> MGVALGATRVIYPAGQKQEQLAVTNNDENSTYLIQSWVENADGVKDGRFIVTPPLFAMKGKKENTLRILDATNNQLPQDRESLFWMNVKAIPSMDKSKLTENTLQLAIISRIKLYYRPAKLALPPDQAAEKLRFRRSANSLTLINPTPYYLTVTELNAGTRVLENALVPPMGESTVKLPSDAGSNITYRTINDYGALTPKMTGVMEHHHHHH;> DLYFNPRFLADDPQAVADLSRFENGQELPPGTYRVDIYLNNGYMATRDVTFNTGDSEQGIVPCLTRAQLASMGLNTASVAGMNLLADDACVPLTTMVQDATAHLDVGQQRLNLTIPQAFMSNRARGYIPPELWDPGINAGLLNYNFSGNSVQNRIGGNSHYAYLNLQSGLNIGAWRLRDNTTWSYNSSDRSSGSKNKWQHINTWLERDIIPLRSRLTLGDGYTQGDIFDGINFRGAQLASDDNMLPDSQRGFAPVIHGIARGTAQVTIKQNGYDIYNSTVPPGPFTINDIYAAGNSGDLQVTIKEADGSTQIFTVPYSSVPLLQREGHTRYSITAGEYRSGNAQQEKPRFFQSTLLHGLPAGWTIYGGTQLADRYRAFNFGIGKNMGALGALSVDMTQANSTLPDDSQHDGQSVRFLYNKSLNESGTNIQLVGYRYSTSGYFNFADTTYSRMNGYNIETQDGVIQVKPKFTDYYNLAYNKRGKLQLTVTQQLGRTSTLYLSGSHQTYWGTSNVDEQFQAGLNTAFEDINWTLSYSLTKNAWQKGRDQMLALNVNIPFSHWLRSDSKSQWRHASASYSMSHDLNGRMTNLAGVYGTLLEDNNLSYSVQTGYAGGGDGNSGSTGYATLNYRGGYGNANIGYSHSDDIKQLYYGVSGGVLAHANGVTLGQPLNDTVVLVKAPGAKDAKVENQTGVRTDWRGYAVLPYATEYRENRVALDTNTLADNVDLDNAVANVVPTRGAIVRAEFKARVGIKLLMTLTHNNKPLPFGAMVTSESSQSSGIVADNGQVYLSGMPLAGKVQVKWGEEENAHCVANYQLPPESQQQLLTQLSAECRLVPRGSWSHPQFEK;> GNKWNTTLPGGNMQFQGVIIAETCRIEAGDKQMTVNMGQISSNRFHAVGEDSAPVPFVIHLRECSTVVSERVGVAFHGVADGKNPDVLSVGEGPGIATNIGVALFDDEGNLVPINRPPANWKRLYSGSTSLHFIAKYRATGRRVTGGIANAQAWFSLTYQ

Uropathogenic Escherichia coli strains use filamentous type 1 pili to adhere to and invade uroepithelial cells. The pilus consists of a flexible tip fibrillum, formed by the adhesin FimH and the subunits FimG and FimF. The pilus rod is a helical assembly of up to 3000 copies of the main subunit FimA, terminated by a single copy of the subunit FimI that anchors the rod to the assembly platform FimD in the outer membrane. The assembly platform FimD in the outer membrane of uropathogenic E. coli is the catalyst of type 1 pilus assembly.

To explore the structural implications of FimI-mediated termination of pilus assembly, we performed a FimD-catalyzed assembly reaction of pilus rods in vitro similar to the one for the FimDHGFAnC complex, except that excess FimICHis was also added at the end of the reaction. Using Ni-NTA affinity chromatography, we separate complexes with a terminal FimICHis subunit from complexes with terminal FimAnC and determine the structure of the FimI-terminated assembly platform at 3.6 Å resolution (map XIII). To identify structural parameters explaining assembly termination by FimI, we next analyzed the interfaces between FimC and FimA (model IV), FimC and FimI (model XIII), and FimC and FimF (PDB-ID 6E1422) in the respective FimD complexes. While the interactions between FimC and the respective subunit (FimA, FimI, FimF) are primarily mediated through backbone hydrogen bonding involving the G1 strand of FimC, differences emerge in the interactions with FimA strand A’. In contrast to FimA and FimF, FimI does not only form hydrogen bonds with the neighboring A1’ strand of FimC, but also with the B1 strand of FimC. Here, Arg25 of FimI additionally interacts with Thr23 and Asn25 of the B1 strand of FimC via hydrogen bonds. In general, the total interface area between FimI and FimC (1739 Å2) is larger than that of FimA and FimC (1562 Å2) or FimF and FimC (1449 Å2) and involves more potential hydrogen bonds (FimI-FimC: 30 H-bonds, FimA-FimC: 21 H-bonds, FimF-FimC: 19 H-bonds). Indeed, we also identified a closed P5 pocket in the FimD-bound FimIC complex. However, when comparing the usher complexes with FimA or FimI as the last incorporated subunit with the usher-tip fibrillum complex (last subunit: FimF, with open P5 pocket), we found that the P5 pocket was closed in the terminal FimA subunit as well as in FimI. In any case, a much stronger binding of FimC to the terminal FimI subunit compared to a terminal FimA due to a larger interface and a higher number of inter-molecular hydrogen bonds appears to be critical for assembly termination by FimI.> MDVQRVGKAGLHRVDSKKQQTAAGVSFSEVMGKQRDEKAYERLQALMSKIDDQGKLLSETRTIEELRKYKELVKEFVGDAVE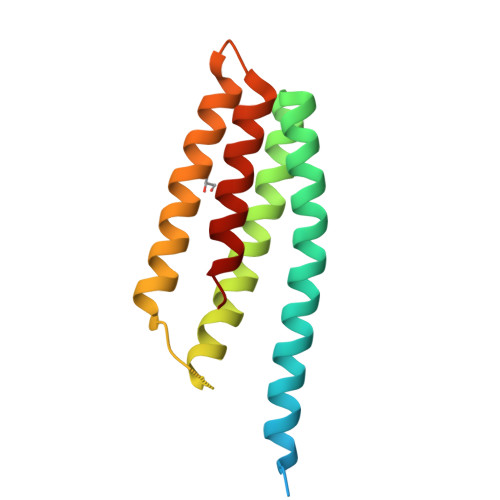LGLRLEERRGFNRRGRTKIYKIVKEVDRKLLDLTDAVLAKEKKGLDILNMVGEIKGLLINIYA> SNAELIISDPTDFEQITHVELGDSGLTGFPPEWRE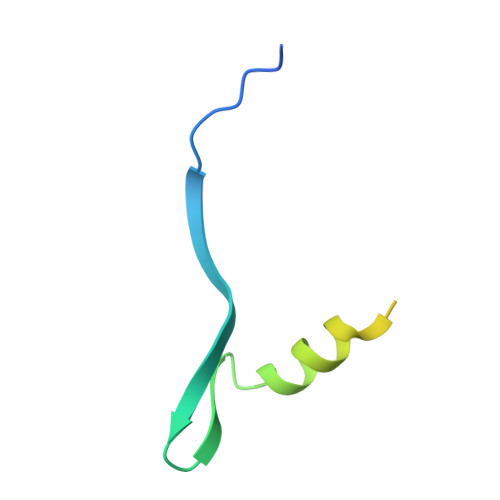KLIKAGLTEAEINTNEDSAKLVAASGISNDNGNRT>MASHRNFTVAIVPGDPHFSVDRDLRGELMPTLYMNQNQWLPSFGPWFISLTDNAMQRRVFPKELKGTVNFQNSTSLKLISHTLTTVASTTADFFADARHLTDTQAALCLVNAYFCQKTSRQLPATPDDLLADLPQKLDLLITQLKQESGPGDFSFTYSNPQERASLAPLNKESRYPTAFFQRHKLHAMMAKAGLFPHNKGTGAPGTAPAMDLVFAITSAMFGSDIPPFSAYQWNLRAGIVALEVFILAYGLLEFGQVARGHPNRRLNLVSLLGPKFQPGALPDPNAPMLKRGQLFSFISEHYIIPTLQANPNAPVSFIFPGIILAALE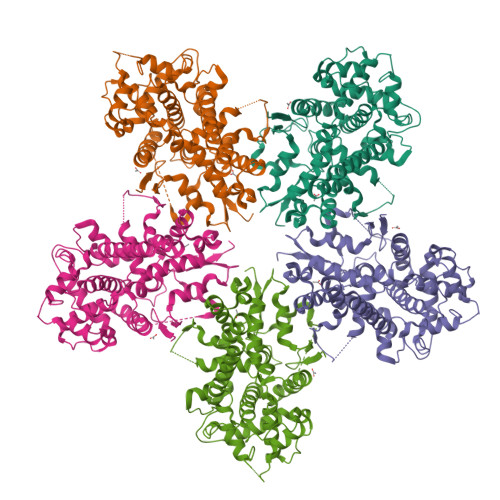ARSTVSHKQPGPFVNLTGSRFNEIFEILNQQLTFRDPLALLQARTALRLATEEGLDVLLSHPSPPTLLQEIIKSQFGGGDDYDRAYFMVLGCLPVVLAVVPAAALEHHHHHHHHH[10x]>SSKQKVDLQSLPTRAYLDQTVVPILLQGLAVLAKERPPNPIEFLASYLLKNKAQFEDRNLERPHRD[4x];> NTLDTLYKEQIAEDIVWDIIDELE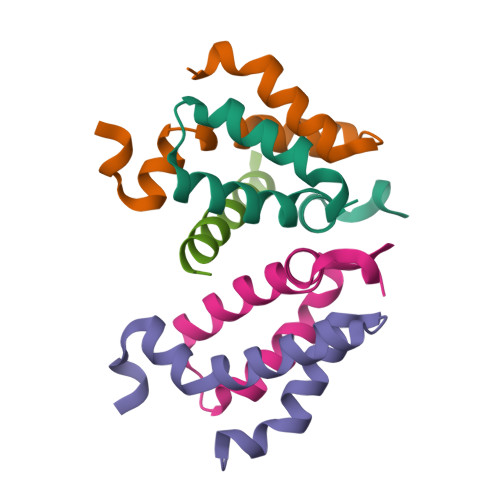QIALQQ> HHHHHHHHHHENLYFQSHMKRSTTDSDLAGDAHNETNKKMKSTEE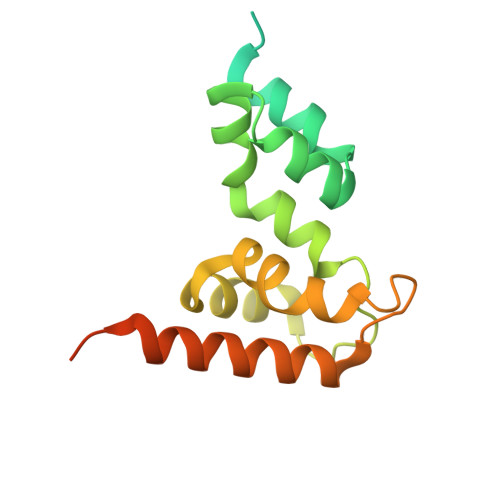EEIGFSNLDENLVYEVLKHVDAKTLAMSSCVSKIWHKTAQDERLWELICTRHWTNIGCGQNQLRSVVLALGGFRRLHSLYLWPLSKPNPRARFGKDELKLTLSLLSIRYYKKMSFTKRPLPESKGGWSHPQFER>GSPGISGGGGGILDSLADFADQVTTPQVVNHVNSNNQAQQMAQKLDQDSIQLRNIKDNVQGTDYEKPVNEAITSVEKLKTSLRANSETVYDLNSIGSRVEALTDVIEAITFSTQHLANKVSQANIDMGFGITKLVIRILDPFASVDSIKAQVNDVKALEQKVLTYPDLKPTDRATIYTK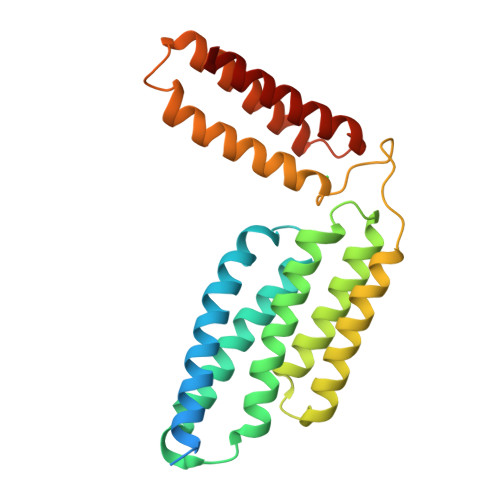SKLDKEIWNTRFTRDKKVLNVKEFKVYNTLNKAITHAVGVQLNPNVTVQQVDQEIVTLQAALQTALK[3x]4-methyl-N-{(1R)-1-[2-methyl-3-(trifluoromethyl)phenyl]ethyl}-7-(piperazin-1-yl)phthalazin-1-amine 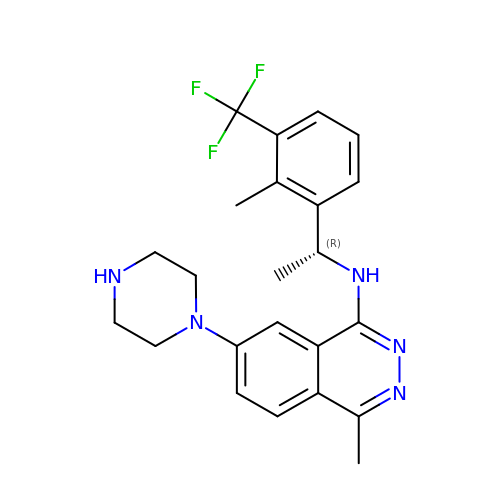| C23 H26 F3 N5 | MJSKXOIIHARCLW-OAHLLOKOSA-N> DITVYNGQHKEAATAVAKAFEQETGIKVTLNSGKSEQLAGQLKEEGDKTPADVFYTAQTATFADLSEAGLLAPISEQTIQQTAQKGVPLAPKKDWIALSGRSRVVVYDHTKLSEKDMEKSVLDYATPKWKGKIGYVSTSGAFLEQVVALS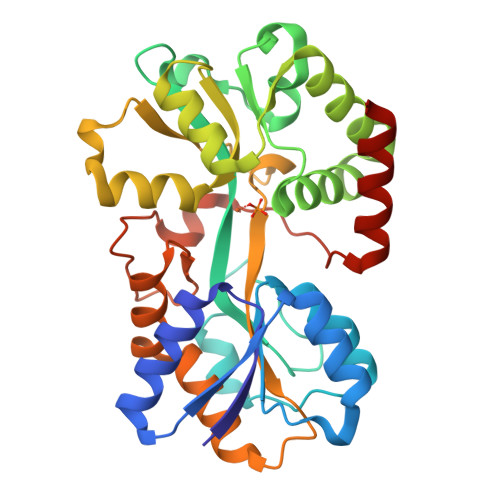KMKGDKVALNWLKGLKENGKLYAKNSVALQAVENGEVPAALINNYYWYNLAKEKGVENLKSRLYFVRHQDPGALVSYSGAAVLKASKNQAEAQKFVDFLASKKGQEALVAARAEYPLRADVVSPFNLEPYEKLEAPVVSATTAQDKEHAIKLIEEAGLK> MTLSTQRRALLAGFGKARGGQWTQEGIAALHSTTTTNAQVETQPDGELAESSADDASRLFQELSRRNRPNSAGTEPGPSPRPVLAQLPAAAELMERAAGTPSSQALYDLPTYLSVTHPHARVEPRNPAYDWRRSPQLEAGGPRRAALLLAVDAHMAAPESREALLRMAQLELAHLWYYQQHAAELPAAASPSASAASAASTATPDAAAAGQRRGGVAKQREAEPAAASTSAAAGDKAQAGAGTGTGAGAGAEAEAGDDDIFAAADRKARERAAAVEAATAAAASSAAKSLGRRGGRLPAELEARVRDMQLRYGMASRDAASVLRLLADSFSRRLPGGGRRLEGEAEAEAAVGLGEAEAEAGGDPTAALTWALSGGGRGGSGGTISGLSRHLAKQAAQAKAADRAIITAMQSLADAVNTASSSSSSATASSSTASSSGSSAYWAAHPALAYDQTLAARAHRQGLAWRAAAEAGPDGAASLSAAITALSASLRRPTSSPTSSASASSPPATPVLDLVLDYLQAKYADLLTAWETAARLREATERVSAAVARARATVPMSAVPPLPPALAAELERSWQNAAAAFRPALLQPLLQPAGSGAAARNSLAAAAASGSPALLQAQSSLTRPLDWAKAKALIEQHYAKQQQAAALAGATAAAEATAAAAAAASAAAAAGSPRGAVEALLQPLLQRAADRHRALLAGGDAAAAEAAAAAAAAAAHGSSTAAAGGAAPSEGAASVVCFRETLTLDASSAYANSSFDSRVTLEFNVDRLAAAEPGLGGAWGARFLERLLATPALPGSGRRIRGGGGSSGMFGRARASPAARAAANAAAYPVDVEHSFCRRTRTAALSTARYGSREANRKLLLEHYNELLRAAALAAAAGASAAV;> MRARLFQSLAIQVAEEGLLTTALSGYACRAFSANGVTKFGFQCSSVSTSAASHEASSSRGSGDQGRVTGGRQERAGRQAPTGSDGPQRADRAKQGYADGGKSRSLFRRDNNPDSGSRGGDGQRGGGKGAGTGSGYSGGSSGQRGGPWQQQQGGRQHDRRGDDRRGGGGGGGPPPMLRDGRDGRDGRGGGGRPPFAPSGPGSGSRAPRAARWDALDVAASNAPQRLLQLVGDPRSGVADDTSSPAFGEVTVELLHHQPSNEVYWYKYAFAGGQPGGRGGHRDGRLSDYSRNLAYVLRAKDPARWSVEALADKFRVRPQRMLAALALKELEAQRLESGALLRGPLSAYSLRVSLADVHLDKASGAPRLRPASAPPAASRELLLGRMLPRVVSATQRTQAALLSALRPHGFDAAALRAALQADVAAVEAAAGELDAAAAAAGGEGAEGGTAAGGVSAYLAPELAACRAAVEAVAAAVEVVVNASPLLQEERQAAALRARVEAALQAGAGQAPAAAAAVAGTGAGAGGGADGNSKDAVPAAAAAAATSPGGGEALEVLLQPLTQDGSGAPLQRFLFSLPPPIRVALLRQLPRLAAQLAAAGVDLQRAGRDAAYRGPLAPAAPAATPAGSKQQQQQRQKQGGAAASTRSGKLPRLTVDVLGFVPVSEAQAEALAAAVESAAAAEAALVAKLEALQVAAGAAPAPAAGAAAAAAAAAATAPSAAELRDARSLLRQYLSTHSMWGELRLAARKAAGHSPDTRGKRRKLEVMAEADPAALTRALQVEAHTQLRRSHDRAAAESLKAGVAAAAATEAAAAAAASGSEAAAKPPTPLSDPAGWDALAAWLDAEVAGRVYARGSGERLVVRLPTYPAFEGYPLSELDKAREGELGALNRLVAARTAAAQWAAFRRDLLFNLGVRGEKLRDNDLPGAPAWPANLRTELTRPVVVYGIGPDGATQYPPVYVAAGDGAKRPLNEQEKVYQERRLPGPRLPYHMGRIRTLPELN;>[3x]XXXXXXXXXXXXXXXXXXMATRQRLMRGIAGLLHQQGQQSSCSQLLMTSAAAASASASSVATGPSHQPALLLRAGSALRGVTTSAPTFNGSLSSLLREEVDYERKNYERPAQISGGPPAPFKLTEAPGDTLLTLTRTFGAEEINVDLHVNSQPSPEYDGEDGDEGISVVAFNVSVAKGDRVLLFECESDGNSVNINHVSLEPKEGLGSESMYSGPVFDELDDNLQGQFGKYLEDRGITAELGEYLRFLIYDKEQREYQNWLSEVEAFVGGK;> MDLIGRGGAPSASALGTDALVLLCGPEAQAGISTCSAAAESAASPQSSCSWVGTAQHSSATRAEAAGPSAPCGPAPLLRNLRTPSQSGRLSGAPPTWISAAAASLGNSPRFAASARCSTADVDVSRSGLEDASALGDCVDRWSTPAATVSGIALLHQYHNHHHNHHHIGHSSSSCGSVASSTSSVPGSAAGSPFPPRPSLPSSATNSSRFLMQSQSQQLRSVSFTAATAAPKAAAKGASAKAGSSSSSGAAAPSPAAAALRTPEWARVPGHLHELQDLYRKRQKRMAALRHGAQVELEAREAVAWKTGGRGRAVAAAAKAALDALPLPPPEDGGKAELAAALAADTTFAAAHEALTGLLRRGVVLDAAEHLAPLLRKAGDAGQLASALGVAAANHLSQAARQLGAHSPRHGPLHAVLVQECRRLKAAAPLVTLWESLHEHGLAPEAADAAAAVRAAVELGDGGAAVRLLMLACMYGEAPLAGAAEAGAVLQLLQQGNPDQAAQLRELLPKLGLRGA;> MRKRELLNEARALVPEGSGWLEAYTRNISPRQLTWRLGKRDSLAAMTEGWQLYQGKFDTVAMAALLRRLRHAQLQDPGFDPLAAQRLLDDLVPRLRSVGLRFGKLRDITAYLHALAKLRSPAPSASSSAASPRAGAAAASLLTQPDALVLDLAVFATRNRTELLHASPQRLATLLWALMRLLPPQLYGSEQLQVVLDRMALASLGRLQNFAPLDLRWAALAFATFGPHGPSSKATATTTAAAAGTRAAAGAGSGPALPEWPRVVRGEAAAAATAGAQGAEDVTARRQSRNARVIKALCDELAARSGNLALPQPEPRDLALAAHALGLVAAASSSAGGAVAPPALLVKAAGVAARSLPALSGEEAVGLVETLAVWGLRQPALLEALRDAAGRWGEGEQAEALRGRLQAAYTRLGVEL;> MRARRSPAINTLDAQLQQADASPASAPSPSSPSSAPLAPSDLDDVLCRHTLRLPKPASTGQEAALRLLSRFNGALPSLRGQTILAKVLSVDSERVTVDTGYNGVAEVPRADVSIAHVHTADGAAPVRPTTSDVRPGDLLRLRVDAPYTPYGDMQLTAVREESEFKRRLAWGELRRAMEAGQPVSGRVLNDCVGGFAVGVAGFVAFLPSAMAARDTTQRVGSLQSFRIVAMDEARRRITLRDAGVAAAGFRRVG;> MLTRLAALGRPAVLDAAAAAVVVAVEPSASASAAWRDGGRDASTSYGVHSLPLAWGAQRRALGALASGCASTAPTPMVASAASAAAQARTGLPFSTAASTPAPVNAPPPPVNAPHLSNTPAELEEAELAGLDMESLMRAIVHPLPLGRVRNGALLAQALGTGAPVVQLENGPGGRDAALFFDPAATLSSTMRALHVIRQVLEKDGHVVVVNSNPRMRPLLREAAHLCLNSNVWFWADDWLPGCLAETDARGGHCPLLSDKAQPNRQIMAEKGLVFRNPLVPDRGNPAAVLGGPAPRLSAADMQRLLAGARSPMGLTHSVYKREQTASHRGCRKALAALTAARTAEARLLLPGSQTGAGRGRFRQPALVVVLDLSYGGEAVREAAARNVPTVALLNGHSDASAVTFPVYASESHLGYHHFFLEWLLRVVNIDPKVLHTLRNAARAAPSAGATGATGATGATGATGATGATGATGATGATGATGATGATGATGATGARAAHAGAGAGAAAAPAAGSGKAAGKAGQQGGRGKR;> MDDMVLVLARNLSGKAKGKPAPKGAPAPPPPPVASSAVTANPATRSAGARIRRNQPRLDPLTLLTPQQRELAESLAHLSRQAAQPPSATAAGADALTPAAEAAADAAAEAAAAPLRGLGEVPLPLRRREVAALVDAALTGAAGGQQVHFQPFVFNDIFQSAPAAATYVAEALESGSAWGRIERFFLAAAEADAGKLVAAVRVEVAGRIGRKADMAATKSWAWGDLRLASLTSKLDYGTAAANTRMGVLGIKVWIRYQPAAAPDLYFPATGGSGLHAPLPAGAAPSMSLDELYAAALERSGSSSSSSSSSSVGGAGGSSTRYGAVGWWSRPAGQQPAANRVHEVFTPEFNPKAGDRLDGYLRRAAESRRVFRSAANREEYMATVGRFLVKQRQAAKARAAAEAYAAALSATKPATIPTTSSSSSSSSANSSAASSVPARPRLGRRPHRPLARFPVEAFSPLGRRGPVLLRWRLQAAAAVGKGKGGNGERRA;> MQRTLRSLATRCAGAITGSTAQTGASGCIKAEAGVSTSALSGLISQDAIHGLCPRGAAFASLASSGVSAAAGAGPASQLRAGAPLSCLWLLALAPSRTGLAATASSSSSCGACGSHSSTSSPFAPLPASAAGLRHYAKAAKGGAAAAPAAPSGPKRPRTSTTKLYSCRNDRLRHTHEQIWPTLQLTEYEQAMFKRNSRLFVVDMGRSLSLRDKFRMGAYEPATAASTGAAAEEAGGAGAGDALVPAAGGASYRRVPYWQARSLLHESNLHLDALGENPRYLRLRRVGSLFATKLQNVRKLRLLLGFQRRGFVQKLYEHSLLARGSDRMWKMVCAMEATLPMTVTRMGLAEDVVGAATAIRNDKIYVNGKQPVMPRKGLLEPGDVVGPAAGGAAYLRKRVARSMEPLASVVTRDYV;> MLRGSILSAQSTGAFSCGAAAVMPSLRSANSLHGSFAASAAFSSPISTTTSCLDVSQNQERGLSTEATGEGESEDDPTYLRGIKTQSGLRNSDGDEEPPDRRKAYEFEPGGRGRGGGGGGGGAPFQRRPADAAAAGTDMLELVATARELFTRNVDSGSGGGGAGGGGGGGGGVGPLPPLPRELREALYGHRWDRVIVDVRRTHTPVRGRGKREEYTAMVATGNMRGVFGLGIGVAESAQLATARAHLDSLSRLAAVPLYRGHTLYTHVDHTFHRLSIRMMPRPAGWGLRCPDLLYELCGLVGLRDVSIRVRGQRGSRFFVAQCFQEALQKQTTPHDGVEATGMYIREVFRGGPGGRLPCGLRRGVDVM;> MPLYELLMLAKPSLPRAEMVALIKGLGDLVYRNGGFVTSLKSFGDQHLAYDLRRPFEKYDRAHIWQMDFVSSVDAIKPLDHGLHVNNTVLRWVLVKRPMSDKSAAAPAAATQAVEAIAQPQR;> XXXXXXXXXXXXXXXXXXXXXXXXXXXXXXXXXXXXXXXXXXXMLSSARRLLATVAEQRALAKADAPAAAAQLRARAGLASVSCCGSTTATITTRLGATGSWRHMSSAADSTSSSSSSSSSQQQQPPAQQQQQPEASTSSAAASSPDGPMSEVVQQLTKASPTGRLLDLFTPSQQQIQTLQRSRGPGRGSRSGTGPAGPAAGTGVQAAEAAAPLTADSDVLEVLMRAVDNCKPLMKVIQSKAGTRVVYQPRPLNPDQSTNFAVKWILQAAQKRRAGAKGVAGAASMAEALAVELLLAAQRKGGARARRDEVHKLALDNRANLRR;> MAAPLLDPLVSKLRQTTATAARAAEVMRAAFPGATHETAGRNTIAVQLPRKDVPTYVMANQRPQPWELLPMKAAAMTQYPNFFNNSCTFFGSIKRDVVNGVPFCLLRPSRLALDMAKVVRNLGIVDGFEVVQRRSRLGAHDFVWLPEQQPQEPEHLYDTSLFRQRLIRLHLRTDLFSRLPGAPGSGAGGPQPASAQLAPAVGLLPLSVKNISKASQPVLMYPRQLEEAAARLPAGVFMCYHPQLGLITDAMAQQYDVPALVAAHVGLPLSQAAAIRGALRVKAAEEAGKELRHVTQLKDWNMMELLRQRMVERRAALEAGMGVGGEVAARLQELREAGLRLRDEASDRVTSALNVAQDLEDGALAWQLVHSRALGAAPGAAAAGVDEGAGGEEQAGAGEGRTSPRGQPRRRR;> MVRGGVATVGPSSLALAASALLGTLPQQTASHSGASLWVFGSRHLAAPAAAGGASNQDRTQPSAKPSAAEPELKLNFSLRPSVLSPLFPAWEQTRQINQRREHLMALLDAHQQLAEGLRITKDGVAASTDGADAGTTSSFAAGGVRAGVTRSARRRARNLQQVASQLRALLDATPGHPRGVTGLPTACPSPAHAVAYCGALEAALASPDAASTGARDFGAVARGDVSPWTHYAKHFAGRYAGAPQLQPLEVIYSRP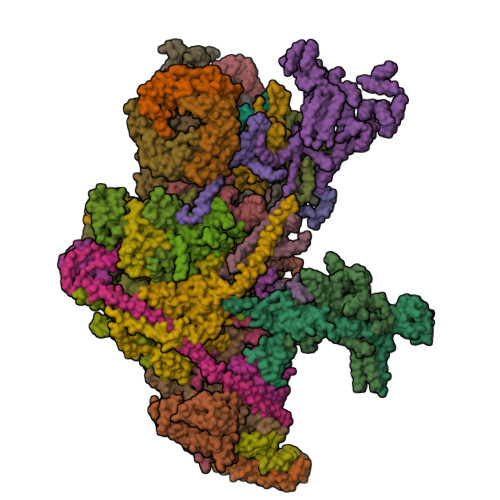DPAEVVRQLRRAAREQEALGISSSGGGSGEAGSGLAFPATSTSPEPAGPHIDLTGVTHARGKRKASAASVQLVPAGGAGITVNGVPLSSYFRDPACREKVLAPLALAGAETAYDVAARVKGGGMMGQAQAIATALARALCVQQPSLGATAGDGGNGEGPLAAMTRWDGRVVERQKPGQAGSRRGFQWVKR;> MQPVVLRGISSLTWQHARGALPSALQQALAASAASSSSSLTAVDCDAGADMQASCSGRGVECARHRLAWGPLSGVAGLSTSARAASPAAAAMPSSSAASAASPAADAAPPGAYSVEIAVQGFEKRYVDMACNTLGDIIILAFAPKSYAALPTGAPSPSDAPVNLAFGPERRDVRLPWRRTRITLIRGPHIDKTGMEQFERREYKSVLTAATNCPQELARLLEAVKLYQFTGVQIKMQLASAQRVDLPADVSALLRGGGGATAASTGSSSSSSSSSSSSSSLVGSPVVXXXXXXXXXXXXXXXXXXXXXXXXXXXXXXXXEIPAPASADLAFAEEVGRVLGVLRPAVWAGLSRRRAVLAGSADHETWLKAAAGGLPPSASATRGAGRGGGAAALPPPAVVAGWDAEAEVAGAAAEGGDAFGRLLRLRLRQQAQLQDAQASTSASGTSTPAAASAAAYGLDPALAARLLARIDADLLHAHEAAAAGLPPPAALAAGTAAAAVAAPPPATAVLDASKMSPAEYAYAVLKYVQYVDSLYESSGAAAAAARGDAALQLAAPALAVRLLQLWWEATTVEFKRALGLPPAEEERRMLERLLELQKKKDELKGAGRGGGR;> MAQASKGLIGALQASLGGLLSTSGRLHGGLGPSAGPAALVSGAWGLSACAAFTRSVATTSAGASATAPAEPGPASTASDAGSGAAQEAEAISSGSNSGGGGFSTGFRKVVSERRAGQLGALEGIVHIQNTLNNIILTLTDKQGLIKTYTSAGVVGYKGSRKSQPVAAEKAAEELARRALKLGYSSVQVRLKGAGSNKQYAVTSLAAAGLTITSLADVTPVPYNGCRLPKKRRV;> MRVWSEVQAAHMATVGQLLGGARKVAKTRKCRIRQLDGSPFKKGICLRVYTTSPKKPNSANRKLAKVQLSNGLKALAYIPGEGHNLQEHSMVLVSGNGVRDLPGVKLRIVRGRYDCAGVKDRKKSSED;> MAQIQRVALFPHATFHIALARVFGLGKSTSLAVSEACGISKDLKVKDVKDSYIQKVTAYIEANFVTGDTLKRQVRENVLEEVAINSRRGVRHTLGLPVSSAQTRSNGVNARKLRPLLLYDTSRR;> MKFRLPQYAYIIGTRGNVKDHMRRMLVEQHEVDRSVFKAVTTDKSVPLEHRLQVQRLFETEVPRDSAANRVVNRCVLTGRARGVHRFARLSRIMIRQLAHSGFLPGVSKASW;> MAGRLLSRLGLIELGASAACAARQPWPATTTAALPMAVLSALHPWRLAWVTPCGALLLSTSSSSGGAAGATEAVSTSAPFVEPSPSTAAGASAGSSSADIAGPSGDSKPDLVEKLLSSDVLGKGERRRYERQALIREFQRHPADTGSPQVMVAVWTHRVRELVKHFDANRKELRPMRELEIMMNQRRRMLTWLRRADFESYAYVISKLGLQDIYTSVGISDRYREGLRPSDPVXXXXXXXXXXXXXXXXXXXKDDSVNRLRFNFHKQYKQKKTNLWQRLRPQLLAEDPVLAAQAVATAAAEKQRQTQQRNATSQRLPAQ;> MEKRQARNSGVRKEDVGWWDPNPAADGNMHLGLNFDRLKYWLTAGAKPTDKVAELLGHAGVLPKVPQPPHYNPRDPKDDTKWRPNEDK;> MGGMEFIGRVVSNRMQKTVVVAVSYVVWVPKYKVYQKRVARHKARDESQASVIGDIVRIRKSRKFSREVSYSVVDTLRKAHVYDPAAAAALVATRDAARAAAAASTGTRAGAAAAGEGQAAQLEGAGFAASGVATSSAGGRSDPWVAEAARRLDASAARLAALRELYEKEVGPGVPLSGAVLAVANSGPGGTGSVRGKAAAAAAGAAEGPGDAKAQQDKQ;> MPACSGLHAHADQQSSLLQLLAQRKGAYSGRPDINQQSRGFASSAGSDNSSSGQQAAGLESERLAPTTRLQDLVAGATERIAQKQVGTLGQLPEQLAAEAASLEHQLASSSGRSGHTHDLDGAGALADRLASAAAAGGPDGRAGGADGAAVTAGQRLLHNKYGYAALGGVVPDGGEMMAAAGPAAVLRSVTAAQPRLHPRRRFQPGQTYEPQDLNPYSSASPESRQRGVGVAVPRPSVAEVLEKADYKNVAFLTRWFLSPAGRLLPRRQTRLPVAVHKHVSRQVRLARHMGLIAGEARLDKTHVQALREVEAAQLLAGRLVAGAEAGAQQQAAAGAGAGAGAAPRQRYNELLDFGA;> MPRSTWKGPYVAVSLLQEVVALARKHPNWWNKGRYIGQKAPEVINTYSRASVILPDFIACRFGVHNGKSFVGMEVQEAMVGHRLGEFAPTKATVQHKAKEVNTQKKKINPKTGKAA;> MNQSTSSLVRLASASFAAIGECTSNLARQLFLSSTLTQFRYTTDSVHQPVNEVQSSSTGPASTICGKGDNRTRRGKIFRGTYREQLPSHGPQLHPYPGGPVVQRPGGGSRGAFRYPGEAPPTAPPGASHTVPPAQR;> MEFWRLVVRPTRRANLVAKLMRDLESGHFAAPKALDVLTQYRTEQLSYSLTGIPRVTLPEKPLIRAFLQKYPEARAEPVALDSFTPPLARQFAQRQLQLMQAGAAREQAFTQAEQELAGRLQALRSRLLGSAATALSEGAQAAVPGPAASGVRGMVELLQQEEQEALDAGLEALASSAQQQQQQLSANSR;> MQSGTVQKLLPSAEMLSALLPGLFVAQTRSKTYTSNVMDETRTKRIIDHFAYHKARKQYRASLHNLYSSWRAELVAKQLADPGAQRRLKAEEAREEAARMAELLREKRVATLVEQVRKAELEHKLAQVQLQRAVRRQEELHRREEARAARYQRLLEASRNWIRQEDLEAAINRALDNPEPFGFVTSLKINRGF;> MTSALLVASRRARQAQGLPRCLLHAIGIHAGTRAEFASVALQEAGTTPSTSGQEQPSSAQLTPAHLRSYYPLNLALLPEAARGSAGAFYTPRDPGHERRGGCKALQQEMEATGRASILYRPIMAALNGAVAAGQQPRLLLTGPAGCGKSLALLGLVEWARQQGWLVVYVPSCLALVRGGYFARRGRGAAGGWDTLTSAQQLLKGVMDAHGPLLQSLPVLPVPGRAARRQQQQQHEPRQADKPAKVEEGQGQGQGQAGGSGLLEEGSGSASGAGGGGGRTLQDVALRGLSSDDNAQLAVDSALQLIRQLQLLGSGAAQPPDSQPGQPPRVLFALDDYNYLYGPTDYGVQPPSASPLQGRRRVLDAGELILARGLRLLESELGTNPVAAAAAGGGAGGVGGAVVVAATTATPALPAPRSLALEVPHTVVEVPGFDEAETAAALAHYAATGAATRAASAAEARHLFALTGGNGRELRAKAGALGVRVG;> MSASTLSRLLPAGSLAWGLPGVLLRSASLLVHHQPCAPSTSGRVQESQLQWSCYYATSHGTGAPKAASTQSSSTTSAASAAASATSAARPAAVSSEAGGDGASSAPFYAGLAARYPDPDTVPDHVMHRLRNTLFGRAVRPRETTGRRALARPLQGKALTDWYWMPPNESPGFHSEEDEYELRRALNRRHTKEAEAEAADTGADKKKKRK;> MAFVELLRSAPKRTLSDLLRKLPNHGVGAIVTRDTWHPESKKYWEVVEVAPSTADPTKLSAWGYQYFKGERQHPAPKRIASVWKYGWLLKEQPGAGLSAAVLQQLSERQAAAQAAGLVAGGSEAAAGTGAAST>[4x]REFNNLTKGLCTI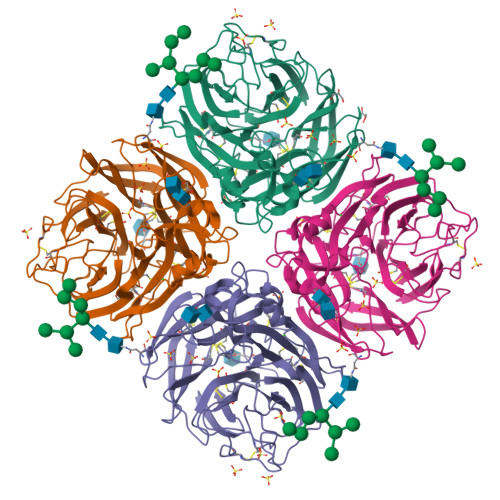NSWHIYGKDNAVRIGEDSDVLVTREPYVSCDPDECRFYALSQGTTIRGKHSNGTIHDRSQYRDLISWPLSSPPTVYNSRVECIGWSSTSCHDGRARMSICISGPNNNASAVIWYNRRPVTEINTWARNILRTQESECVCQNGVCPVVFTDGSATGPAETRIYYFKEGKILKWEPLTGTAKHIEECSCYGEQAGVTCTCRDNWQGSNRPVIQIDPVAMTHTSQYICSPVLTDNPRPNDPTVGKCNDPYPGNNNNGVKGFSYLDGGNTWLGRTISVASRSGYEMLKVPNALTDDRSKPTQGQTIVLNTDWSGYSGSFMDYWAEGECYRACFYVELIRGRPKEDKVWWTSNSIVSMCSSTEFLGQWNWPDGAKIEYFL> AATLISAADYSPTEKILLNCGGGASNLTDTDNRIWISDVKSKFLSSSSEDSKTSPALTQDPSVPEVPYMTARVFRSPFTYTFPVASGRKFVRLYFYPNSYDGLNATNSLFSVSFGPYTLLKNFSASQTAEALTYAFIIKEFVVNVEGGTLNMTFTPESAPSNAYAFVNGIEVTSMPDMYSSTDGTLTMVGSSGSVTIDNSTALENVYRLNVGGNDISPSADTGLYRSWYDDQPYIFGAGLGIPETADPNMTIKYPTGTPTYVAPVDVYSTARSMGPTAQINLNYNLTWIFSIDSGFTYLVRLHFCEVSS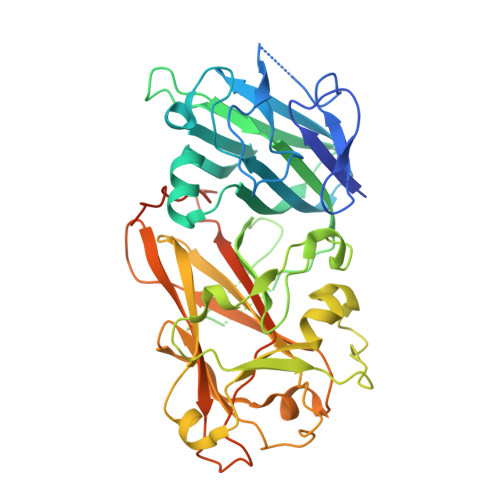NITKINQRVFTIYLNNQTAEPEADVIAWTSSNGVPFHKDYVVNPPEGNGQQDLWLALHPNPVNKPEYYDSLLNGVEIFKMNTSDGNLAGTNPIPGPQVTADPSKVLRPTTRKSKSNTAIIA> MRVLITGCGSRGDTEPLVALAARLRELGADARMCLPPDYVERCAEVGVPMVPVGRAVRAGAREPGELPPGAAEVVTEVVA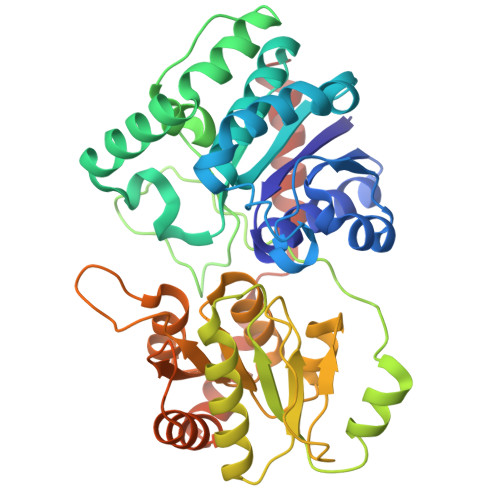EWFDKVPAAIEGCDAVVTTGLLPAAVAVRSMAEKLGIPYRYTVLSPDHLPSEQSQAERDMYNQGADRLFGDAVNSHRASIGLPPVEHLYDYGYTDQPWLAADPVLSPLRPTDLGTVQTGAWILPDERPLSAELEAFLAAGSTPVYVGFGSSSRPATADAAKMAIKAVRASGRRIVLSRGWADLVLPDDGADCFVVGEVNLQELFGRVAAAIHHDSAGTTLLAMRAGIPQIVVRRVVDNVVEQAYHADRVAELGVGVAVDGPVPTIDSLSAALDTALAPEIRARATTVADTIRADGTTVAAQLLFDAVSLEKPTVPALEHHHHHH> MKEFYLTVEQIGDSIFERYIDSNGRERTREVEYKPSLFAHCPESQATKYFDIYGKPCTRKLFANMRDASQWIKRMEDIGLEALGMDDFKLAYLSDTYNYEIKYDHTKIRVANFDIEVTSPDGFPEPSQAKHPIDAITHYDSIDDRFYVFDLLNSPYGNVEEWSIEIAAKLQEQGGDEVPSEIIDKIIYMPFDNEKELLMEYLNFWQQKTPVILTGWNVESFAIPYVYNRIKNIFGESTAKRLSPHRKTRVKVIENMYGSREIITLFGISVLDYIDLYKKFSFTNQPSYSLDYISEFELNVGKLKYDGPISKLRESNHQRYISYNIIAVYRVLQIDAKRQFINLSLDMGYYAKIQIQSVFSPIKTWDAIIFNSLKEQNKVIPQGRSHPVQPYPGAFVKEPIPNRYKYVMSFDLTSLYPSIIRQVNISPETIAGTFKVAPLHDYINAVAERPSDVYSCSPNGMMYYKDRDGVVPTEITKVFNQRKEHKGYMLAAQRNGEIIKEALHNPNLSVDEPLDVDYRFDFSDEIKEKIKKLSAKSLNEMLFRAQRTEVAGMTAQINRKALINGLAGALGNVWFRYYDLRNATAITTFGQMALQWIERKVNEYLNEVCGTEGEAFVLYGDTDSIYVSADKIIDKVGESKFRDTNHWVDFLDKFARERMEPAIDRGFREMCEYMNNKQHLMFMDREAIAGPPLGSKGIGGFWTGKKRYALNVWDMEGTRYAEPKLKIMGLETQKSSTPKAVQKALKECIRRMLQEGEESLQEYFKEFEKEFRQLNYISIASVSSANNIAKYDVGGFPGPKCPFHIRGILTYNRAIKGNIDAPQVVEGEKVYVLPLREGNPFGDKCIAWPSGTEITDLIKDDVLHWMDYTVLLE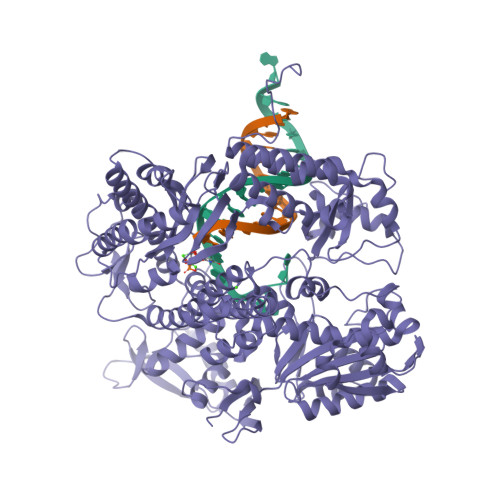KTFIKPLEGFTSAAKLDYEKKASLFDMFAF>HPETLVKVKDAEDQLGARVGYIELDLNSGKILESFRPEERFPMMSTFKVLLCGAVLSRIDAGQEQLGRRIHYSQNDLVEYSPVTEKHLTDGMTVRELCSAAITMSDNTAANLLLTTIGGPKELTAFLHNMGDHVTRLDRWEPELNEAIPNDERDTTMPVAMATTLRKLLTGELLTLASRQQLIDWMEADKVAGPLLRSALPAGWFIADKSGAGERGSRGIIAALGPDGKPSRIVVIYTTGSQATMDERNRQIAEIGASLIKHW[2x];>AGVMTGAKFTQIQFGMTRQ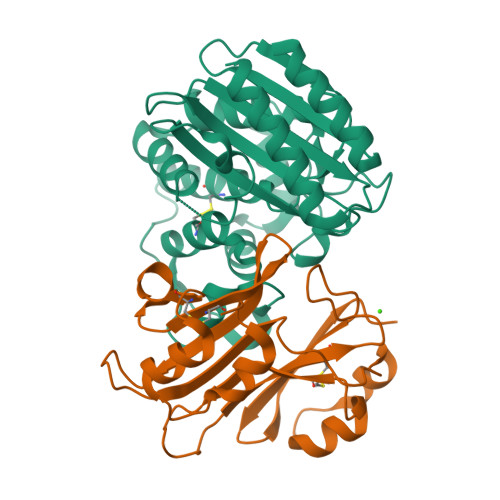QVLDIAGAENCETGGSFGDSIHCRGHAAGDYYAYATFGFTSAAADAKVDSKSQEKLLAPSAPTLTLAKFNQVTVGMTRAQVLATVGQGSCTTWSEYYPAYPSTAGVTLSLSCFDVDGYSSTGFYRGSAHLWFTDGVLQGKRQWDLV[2x]> MEKYREIHQRVKEIPPGGASALECLDLLDRLYAVRHDVVDQMIKHDWSDNKDMERPIGQVLLMAGVPNDIIQGMEKKVIPTSPSGQILKSFFRMTPDNYKITGALIEFIEVTVTADVAKGIREAKLKYESGLQFIESLLSQEHKKGNINQVYKITFDVVAVKTDGSNISTQWPSRRNDGVVQHMRLVQADINYVREHLIKPDERASLEAMFNLKFHVGGPKLRYFNIPDYKPQSLCQPEITNLIQYCKHWLTEDHDFVFKEVTGNNVMSSFENNEDVYMSRYKESRKPRNFLLIQGSIQGPYLPSTISSDQCDTRIGCLEVLKVHPETPVQAIAVDMAYKYMELNRDEIINYYNPRVHFQATQSVKEPGTFKLGLSQLNPMSKSILDQVGKHKSEKGLFGEPLESINISSQIQQNECSRIIESILSNLEINVGEVTMNLANPRKTTGVDELLGKFYENELSKYLISILRKTAAWHIGHLIRDITESLIAHAGLKRSKYWSIHAYDHGGVILFILPSKSLEVVGSYIRYFTVFKDGIGLIDEENLDSKVDIDGVQWCFSKVMSIDLNRLLALNIAFEKALLATATWFQYYTEDQGHFPLQHALRSVFSFHFLLCVSQKMKICAIFDNLRYLIPAVTSLYSGYELLIEKFFERPFKSALEVYLYNIIKALLISLAQNNKVRFYSKVRLLGLTVDHSTVGASGVYPSLMSRVVYKHYRSLISEATTCFFLFEKGLHGNLNEEAKIHLETVEWARKFEAKERKYGDILMREGYTIDAIRVGDVQVEQQLFCQEVVELSAEELNKYLQAKSQVLSSNIMNKHWDKPYFSQTRNISLKGMSGALQEDGHLAASVTLIEAIRFLNRSQTNPNVIDMYEQTKQHKAQARIVRKYQRTEADRGFFITTLPTRVRLEIIEDYYDAIARVVPEEYISYGGDKKILNIQTALEKALRWASGSSEITTSTGNVIKFKRRLMYVSADATKWSPGDNSAKFKRFTQALYDGLSDEKLKCCVVDALRHVYETEFFMSRKLHRYIDSMDEHSEAVQDFLDFFKGGVSATVKGNWLQGNLNKCSSLFGAAVSLLFRRIWAELFPELECFFEFAHHSDDALFIYGYLEPEDDGTDWFLYVSQQIQAGNYHWHAVNQEMWKSMFNLHEHLLLMGSIKVSPKKTTVSPTNAEFLSTFFEGCAVSIPFIKILLGSLSDLPGLGFFDDLAAAQSRCVKAMDLGASPQLAQLAVVICTSKVERLYGTADGMVNSPVAFLKVTKAHVPIPLGGDGSMSIMELATAGIGMADKNILKQAFYSYKHTRRDGDRYVLGLFKFLMSLSEDVFQHDRLGEFSFVGKVQWKVFTPKNEFEFYDQFSQSYLKSWTNQHPVYDYIIPRGRDNLLVYLVRKLNDPSIVTAMTMQSPLQLRFRMQAKQHMKVCKLDGEWVTFREVLAAADSFATKYNPTEKDLDLFNTLVSCTFSKEYAWKDFLNEVRCEVVPTKHVHRSKIARTFTVREKDQAIQNPITAVIGYKYASTVDEISDVLDSSFFPDSLSADLQVMKEGVYRELG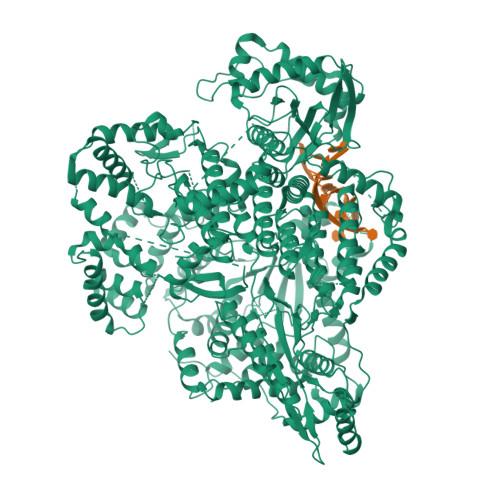LDIGLPEVLKRIAPLLYKAGRSRVVIVEGNVEGTAESICSYWLRSMSLVKTIKVRPKKEVLRAVSLYSTKENIGLQDDVAATRLCIEVWRWCKANDQNVNDWLNALYFEKQTLMDWVERFRRKGVVPVDPEIQCIALLLYDVLGYKSVLQMQANRRAYSGKQYDAYCVQTYNEETKLYEGDLRVTFNFGLDCARLEIFWDKKEYILETSITQRHVLKLMMEEVTQELLRCGMRFKTEQVSHTKSLVLFKTESGFEWGKPNVPCIVFKHCALRTGLRTKQAINKEFMINVQADGFRAIAQMDVESPRFLLAHAYHTLRDVRYQAVQAVGNVWFQTNQHKLFINPIISSGLLENFMKGLPAAIPPAAYSLIMNKAKISVDLFMFNELLALVNPRNVLNLDGIEETSEGYSTVTSISSRQWSEEVSLMADDNIDDEEEFTIALDDIDFEQINLDEDIQHFLQDESAYTGDLTIQTEEVEVKRIRGVTRVLEPVKLIKSWVSKGLAIDKVYNPIGIVLMARYMSKNYDFSKIPLALLNPYDLTEFESVVKGWGETVNDRFLEVDNDAQRLIREKNILPEDILPDSLFSFRHVDVLLKRLFPRDPVSSFY> MLVELLEFTPLSFIDDVINITNQLLYKGVNGVDKAFSQTRFAKKAPQEIE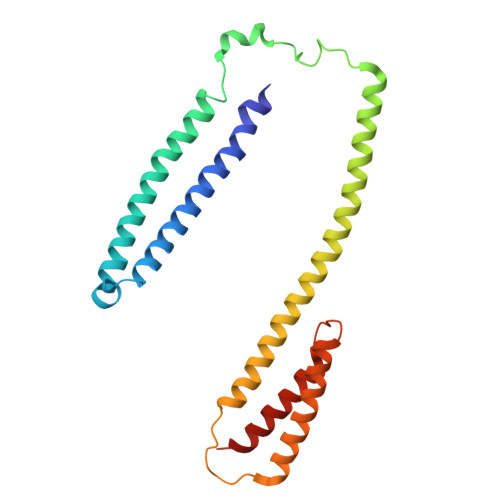EGLHKFEVLFESVVDRYYDGFEVYTLRNIFSYPPELKGYMRTFGKDVDYSITTEQDAAMDQAIQEAAEKLVVKMQLRRDLRMRLSRKREKKTEIEKHLERISFLNKVPENWQVTLPETTDFLLDQLGNLQHAVKRVVEASPTVHSREVDERITYLEKGYERLSNP ACETONITRILE | C2 H3 N | 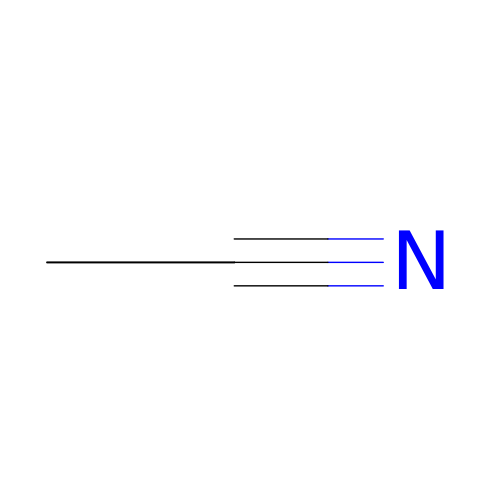WEVYAHXRMPXWCK-UHFFFAOYSA-N> MKYSQCLKGEVVMIPALAKKILHVTVGTLLVSSAASMMVYLNSMCHMAANSKTQQIQGDDNKDDKFPLASISKVVTTLWAVDRLGPDYRFKTKLHVTPTANGSYDIHIEGSRDPLFGRNMSYFLISELNRMKITKIEKLTFDENFLLAWLAEEKPMIGGTTPKYDTVEQQASIVRATLTSSFATAISPGYYTILKTKAARIGVQMSNRPKIDVRTISFVKKAEFQKNEKSTTMVLMSAPLKTILKRMNNQSNNYIADNLYWNLGGTEAFNAYIAGKMQADTSDIEFHNGSGNNEGSVAKPVYNEATCEMMIKVLYSLDKSLSAKGYDLSDVMAVAAKDKASTVGSYGGVMAGSTTAKTGSVNKAKTLMGSVSTKNGEIYFAVLMHTDYDKSRSDWGVASQQIKNKVSQLINQNGGPKAIKYTEQLPLPFDKYSYLTKANTITTEKK;> MKKSYLLAALIFFLAGLLHGTAFAMSGKSSKALNEAAEQGDLAKVKNLVQKNKIDLNAQDETGMTPLMNAAMGGNLDIVKFLLSKKVNLELKNNGGETALAFAVTNDAYDVAEELIKAGANVDIIVAGDEGDTLFMRAAQNNKKTAESILAKNKSLINKANTLGETALFAVARYGTPADIDFLIKKGADLKLKNKKGQTALDVAKEASNQDTAKALSKKKLEHHHHHHHH

Here we show that Bdellovibrio bacteriovorus utilizes a small ankyrin repeat protein, Bd3460, to protect itself from endopeptidase activities during entry of prey. We demonstrate that endopeptidase complexation by Bd3460 prevents cell wall decrosslinking, and that both the Bd0816 and Bd3459 targets bind this self-protection protein via a common epitope. Previously, we assigned prey cell rounding to the action of two secreted Bdellovibrio peptidoglycan DD-endopeptidases, Bd0816 and Bd3459, that act to modify the invaded cell wall via hydrolysis of the structural 3-4 peptide crosslinks6. In summary, we conclude that we have identified and characterized the first ever self-protection protein encoded by predatory bacteria—ankyrin repeat protein Bd3460 from Bdellovibrio inhibits the prey wall decrosslinking enzymes Bd3459/Bd0816 and in doing so protects the predator from the shape transition that this catalyses in prey.

We next utilized a modified version of our original Bd3459 construct (starting post signal peptide with K38 mutated to become the new N-terminal methionine) that represents a more ‘native' signal peptide-processed form of the DD-endopeptidase6. This version (hereafter simply referred to as Bd3459), was co-expressed with the exported domain of Bd3460 and the structure of this complex determined to 1.36 Å resolution. The Bd3459:Bd3460 interaction reveals that AR1-3 of the self-protection protein are located over the endopeptidase active site cleft, whereas AR4-6 contact the final α-helix of the transpeptidase domain (α9). The Bd3459:Bd3460 interface buries 2372 Å2 of surface area, and is largely polar in nature; 13 hydrogen-bonds, 1 salt bridge, 125 non-bonded contacts; indicating complexation largely via shape complementarity. Upon comparison with our structures of the uncomplexed proteins, Bd3459 does not alter in conformation upon binding, whereas Bd3460 undergoes further flexation around the region between AR4-AR5. This observation explains the 4+2 arrangement of the repeats, such that the gap between AR4 and AR5 allows Bd3460 to undergo an induced fit and contact a patch of Bd3459 around the 346-351 loop and C-terminal end of helix α9. To the best of our knowledge, this significant conformational rearrangement following ARP target complexation is unique. The protein complexes show that the interaction face involves the signal peptide cleavage site for Bd3459/Bd0816, hence binding may potentially be strongest to the mature form of these enzymes and thus not interfere with secretion and/or processing by signal peptidase, with Bd3460 forming protective complexes only in the periplasm.> GSHMKNSVSVDLPGSMKVLVSKSSNADGKYDLIATVDALELSGTSDKNNGSGVLEGVKADASKVKLTISDDLGQTTLEVFKSDGSTLVSKKVTSKDKSSTEEKANEKGEVSEKIITRADGTRLEYTGIKSDGSGKAKEVLKGYVLEGTLTAEK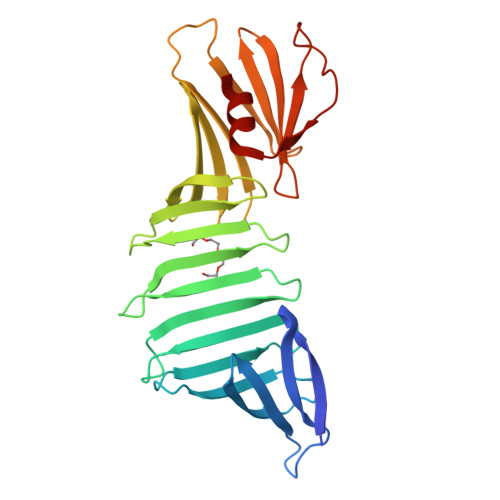TTLVVKEGTVTLSKNISKSGEVSVELNDTDSSAATKKTAAWNSGTSTLTITVNSKKTKDLVFTSSNTITVQQYDSNGTSLEGSAVEITKLDEIKNALK>[2x]GSHGSGSMIEYIIGALGLIIASVQDFRSREIEDYIWIFLAVFGVLFAIYSSITLLDYSILINSISGFVICFILGYMMFLSGIGGGDGKMLIGLGA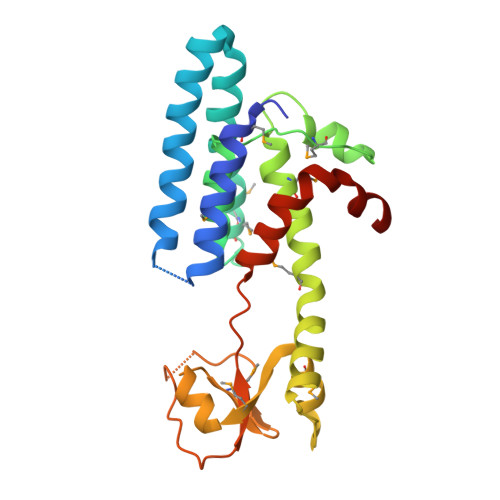LVPKFQMPIYTSLGTLLNLNYVPTFPIMVFINGIFFMVFLPFVILFRNILNGARPKTGKEFILMFFGEKMKVNVAKEQKRLIMGQNDKINFFPAADDEDFSKYSNNEEIWVTPQIPLIIPITLSYLVTPIIGDRILDFLIPF> MSSLPPAIFLMGPTAAGKTDLAMALADALPCELISVDSALIYRGMDIGTAKPSRELLARYPHRLIDIRDPAESYSAAEFRADALAAMAKATARGRIPLLVGGTMLYYKALLEGLADMPGADPEVRAAIEAEAQAEGWEALHRQLAEVDPESAARIHPNDPQRLMRALEVYRLGGVSMSDLRRRQSAEKADFDASGRNQLPYTVAQ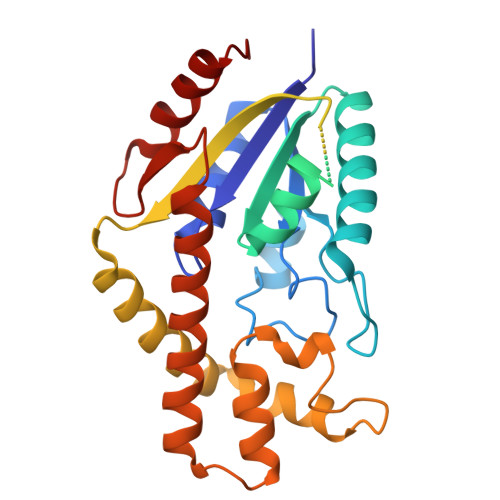LAIAPEQRQVLHARIAQRFRQMLEQGFIAEVEALHARSDLHAGLPSIRAVGYRQVWDYLDGKLSYAEMTERGIIATRQLAKRQFTWLRSWSHLHWMDSLAGDNLPRALRYLKTVSILA>[2x]DWSWYAPSELVAKQIANVPFNVLAGTPIKASVHLRYDPSLVSGLKDQLFVGNNASIMGARLLYLPSFGISTTVLDGLSMAANQLYAYVRKSNSGAKVYE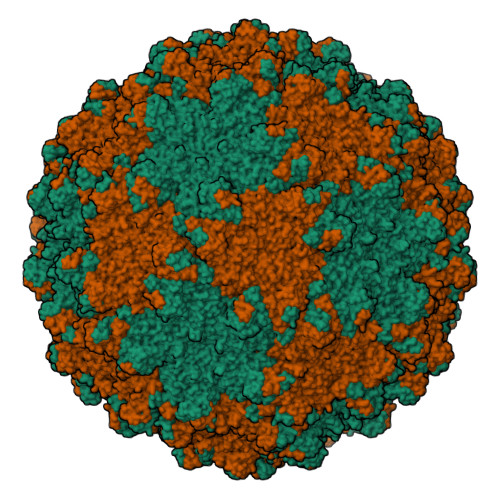APDLMMTVLAIQEAYRVLFEIRRAITFANYWNFWNKYLPKQVFEQLLAIDFDDLMSNKANYCAQFNLMAQKINTFALPKYFKSILRMAYVSSNIFMDSDAVTGQMYAFVSSGYYRYSATTSESGTSLVYRDWPVGAAMPRKLNRLFTVLRELLDAIYGDADAQTMFGDIYKAFGSDGLYSIAEISVDETSTPVFDVDILAQIENCTILEANAGLAWTLDSCNVTQSKGQVLLWQPTGTITSSDNTEHIAGDIAVALGDRVLNSHIMEPQYSDVLEWTRLMATIEFDKASVTSSEKVTFKVTSCGAELIRNVLYFKNVWNDAAEDASQRVITYFSHFSQITVTNATDDPTSAYGLMSNTLDFTQLDWHPIIYVTETSVHNVANLNSILIGGDLKRPTVITTDVVKRINSAANYALYYSANLLSNIST> MAGGLSQLVAYGAQDVYLTGNPQITFFKTVYRRYTNFAIESIQQTINGSVGFGNKVSTQISRNGDLITDIVVEFVLTKGGNGGTTYYPAEELLQDVELEIGGQRIDKHYNDWFRTYDALFRM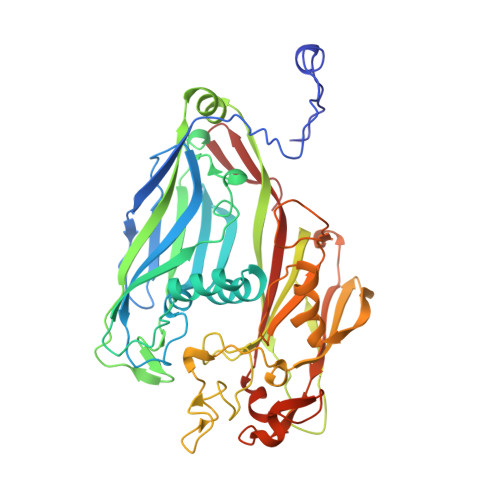NDDRYNYRRMTDWVNNELVGAQKRFYVPLIFFFNQTPGLALPLIALQYHEVKLYFTLASQVQGVNYNGSSAIAGAAQPTMSVWVDYIFLDTQERTRFAQLPHEYLIEQLQFTGSETATPSATTQASQNIRLNFNHPTKYLAWNFNNPTNYGQYTALANIPGACSGAGTAAATVTTPDYGNTGTYNEQLAVLDSAKIQLNGQDRFATRKGSYFNKVQPYQSIGGVTPAGVYLYSFALKPAGRQPSGTCNFSRIDNATLSLTYKTCSIDATSPAAVLGNTETVTANTATLLTALNIYAKNYNVLRIMSGMGGLAYAN>[2x]SNAEHPVDGTPVRFYDALTKARGSAVDESYLTFGVLNEKQPGFSWLRVAYGLDPSEERMRLLLHSQRALRNVLLDSVDFSRAKSVWDFGCGYASDIIALGERHSHLKLHGHTLSSEQAELGLRKIEARGLGGRVQVL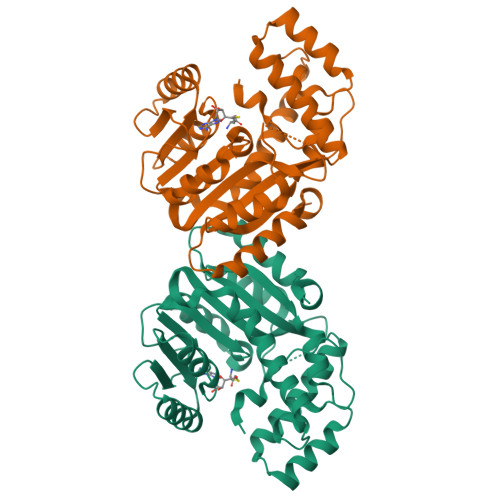RRDSSKDAPLESAYDVILGFEVATHIKEKRSLFQNLSSHLREGGFMLLADFIANSGSGVDVQDIASYNVTPSQWVELLSEHGLRLVECVDVSQEVANFLFDADFDANLTQLETSVGISAIEKRNYQAMRNFGAALERKILSYVLFIAQKDSHVRSTYLRHINQKWVEAPAPYAARELM(3BETA)-3-HYDROXYPREGN-5-EN-20-ONE 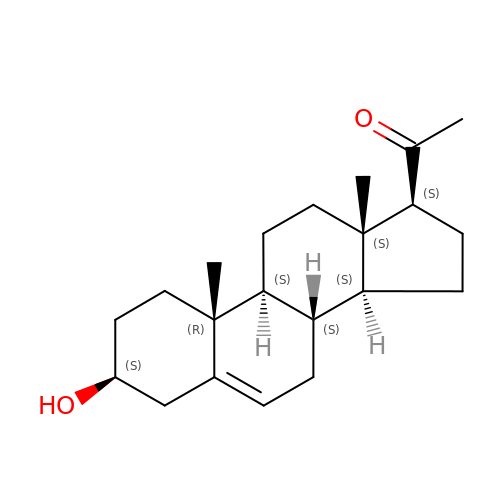| C21 H32 O2 | ORNBQBCIOKFOEO-QGVNFLHTSA-N> ANSLEPEPWFFKNLSRKDAERQLLAPGNTHGSFLIRESESTAGSFSLSVRDFDQNQGEVVKHYKIRNLDNGGFYISPRITFPGLHELVRHYTNASDGLCTRLSRPCQT;> PEPWFFKNLSRKDAERQLLAPGNTHGSFLIRESESTAGSFSLSVRDFDQNQGEVVKHYKIRNL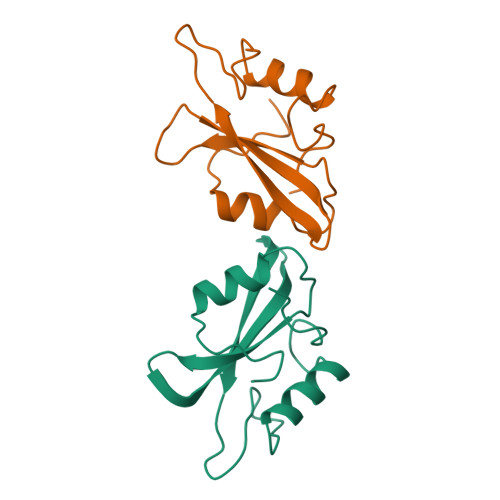DNGGFYISPRITFPGLHELVRHYTNASDGLCTRLSRPCQT> MQKYRLYEKDGSPVQDFNRFVKGWLDIEFGLKEHQPPKVFDTIRDKYNEAIEAVVLSGVAPRTAHKAALSTLTELLFGHDLAKELSARLDIQPIGVGGFRSAHSQAFAKNVGENFVNLMVYALACILKDNDDVLVDKGLPPHLKKALTLSRECRIKDTLREIKIPIEGDLCVFSRSNHCNAIVISAKTRLKEVFHIGTMWALFSDVAKDEYCLNKWGLKVESSESLKDTMYVFATADMINKDGARSQGCDVERETPRNLIAMDASFFDYVFVSKMGIGHVSSDLSLKYGRESLFHELGCIIDMIEQKFDILL

PfoI belongs to the CCGG-family and cleaves the 7 bp sequence 5′-T|CCNGGA ("|" designates cleavage position). The overall fold of PfoI monomer represents a typical PD…D/ExK nuclease fold with the structural core made of central four-stranded β-sheet surrounded by α-helices (50–52). The PfoI monomer is composed of an N-terminal α-helical subdomain (residues 1-131, colored pink-yellow and blue-green in Figure 1B and C) and the C-terminal subdomain (residues 132–312) that bears PD…D/ExK core (colored orange and cyan in Figure 1B and C). Structures and mutagenesis indicate that PfoI features a permuted E…ExD…K active site that differs from the consensus motif characteristic to other family members.

We solved the crystal structure of apo-PfoI at 2.6 Å resolution. Interestingly, the apo-PfoI crystals grow only in the presence of the specific oligoduplex that was not present in the crystal. In the crystal only one protein chain is present in the asymmetric unit; the dimer is obtained by applying crystallographic symmetry. In the apo-PfoI crystal structure two monomers related by the crystallographic symmetry (the symmetry operator: y-1,x+1,-z) form a dimer. The dimer has the U-shape typical for other related REs. The dimer interface as calculated by PISA extends over ∼1890 Å2. Three different regions of the C-subdomain contribute to the dimer interface: a β-hairpin (residues 151–167), α-helix (residues 192–218) of the conserved RE core, and a region including residues 255–266, 278–282 and 288–293 that interacts with the β-hairpin of the other subunit. In total, the interface contains 26 hydrogen bonds and two salt bridges. Residues 239–249 are disordered in the apo-PfoI structure. Residues 78–111 are swapped between two monomers of PfoI–DNA complex, whereas in the apo-PfoI structure this structural element is bound to the same subunit.>[2x]GSLNEVENTAQKFCVKLDVAAFKPEELKVNLEGHVLTI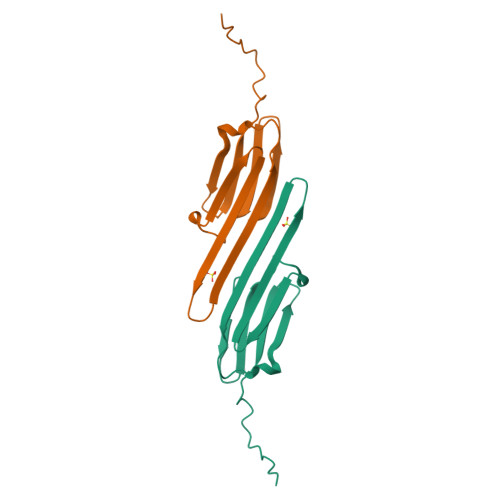EGHHEVKTEHGFSKRSFTRQFTLPKDVDLAHIHTVINKEGQMTIDAPKTGSNTTVRALPIHTSAGHAVTQKPSSTTTTGKH5-IODOURIDINE-5'-MONOPHOSPHATE | C9 H12 I 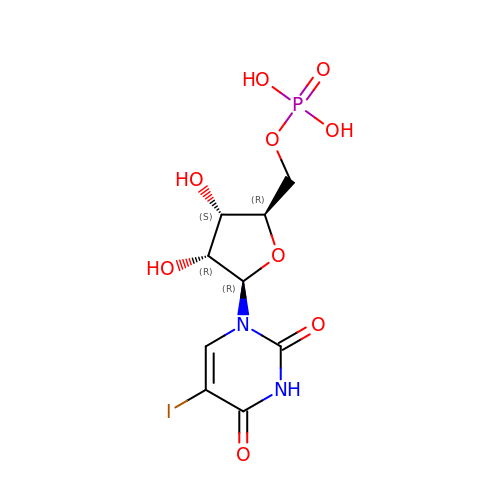N2 O9 P | HXJLWCWPONZYNP-UAKXSSHOSA-N> MRGIVTIDGPSASGKSSVARRVAAALGVPYLSSGLLYRAAAFLALRAGVDPGDEEGLLALLEGLGVRLLAQAEGNRVLADGEDLTSFLHTPEVDRVVSAVARLPGVRAWVNRRLKEVPPPFVAEGRDMGTAVFPEAAHKFYLTASPEVRAWRRARERPQAYEEVLRDLLRRDERDKAQSAPAPDALVLDTGGMTLDEVVAWVLAHIRR

NMP kinases include adenylate kinase (AMPK), cytidylate kinase (CMPK), guanylate kinase, and thymidylate kinase, which catalyze conversions of respective NMPs to the corresponding nucleoside diphosphates. NMP kinases are bi-substrate enzymes that bind both substrates simultaneously to catalyze phosphoryl transfers. In this research, we determined structures of the ligand-free-, CMP-bound, CDP-bound, and ADP-CDP-bound forms of CMPK from an extremely thermophilic eubacterium, Thermus thermophilus HB8 (ttCMPK). The overall structure of ttCMPK consists of three domains: CORE domain, NMP-binding domain, and LID domain.

We also solved another structure of a CMP-bound form, which was crystallized under a different condition. In contrast to the CMP "open" complex, this complex showed a closed conformation. We designate this complex as the CMP "closed" complex. Comparison of the overall structure of the CMP "closed" complex with the ligand-free form revealed large shifts in the position of the NMP-binding domain and LID domain relative to the CORE domain. The RMSD value between these two structures (196 Cα atoms) was 6.56 Å. These shifts lead to closure of the substrate-binding cleft, where CMP is bound. Therefore, it can be indicated that the closure of the cleft occurs by rotation of the NMP-binding domain around the α6 helix as an axis. It should be mentioned here that crystallization condition for the CMP "closed" complex contained AMP-PCP, an ATP analogue. No electron density of AMP-PCP was found, and no significant movement of the side chains was observed in the ATP-binding site. Furthermore, three residues from the CORE domain interact with CMP in the CMP "closed" complex. Lys15 and Arg126 interact with the α-phosphate group, and Asp127 interacts with the amino group of N4 from cytosine.> MLSDMSLIATLSFFTLLPFLVAAGTCYIKFSIVFVMVRNALGLQQVPSNMTLNGIALIMALFVMKPIIEAGYENYLNGPQKFDTISDIVRFSDSGLMEYKQYLKKHTDLELARFFQRSEEENADLKSAENND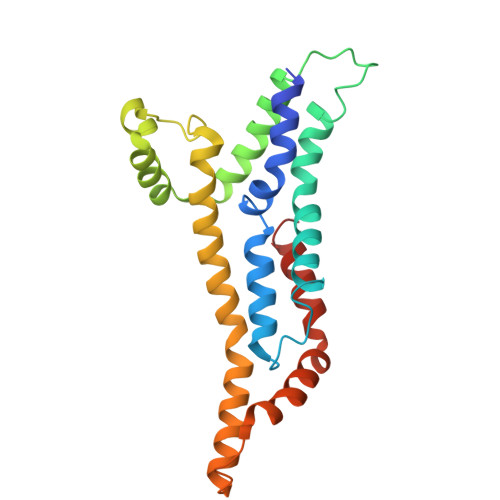YSLFSLLPAYALSEIKDAFKIGFYLYLPFVVVDLVISSILLALGMMMMSPITISVPIKLVLFVALDGWGILSKALIEQYINIPA>SYYIAPRFLDKLAVHITKNFLNIPGVRVPLILGIHGRKGEGKTFQCELAFEKMGIEVTLISGGELESPDAGDPARLIRLRYRETAELIKVRGKMCVLMINDLDAGAGRFDEGTQYTVNTQLVNATLMNIADNPTDVQLPGSYDSNPIRRVPIIVTGNDFSTLYAPLIRDGRMEKFYWEPNRDDKVGIVGGIFAEDGLSQREIEQLVDTFPKQSIDFFSALRSRIYDIQIRDFIHKVGFERISLRVVNSLEAPPEFKKPDFSLA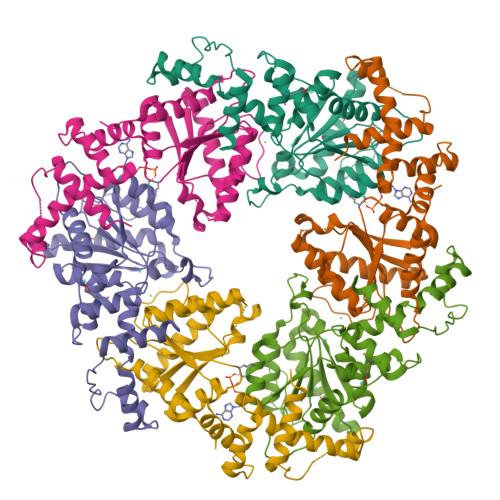HLIESGNLVLGEQQRVDNSQLVDEYNR[2x]> MAAEEGVASAASAGGSWGTAAMGRVLPMLLVPVPAEAMGQLGSRAQLRTQPEALGSLTAAGSLQVLSLTPGSRGGGRCCLEGPFWHFLWEDSRNSSTPTEKPKLLALGENYELLIYEFNLKDGRCDATILYSCSREALQKLIDDQDISISLLSLRILSFHNNTSLLFINKCVILHIIFPERDAAIRVLNCFTLPLPAQAVDMIIDTQLCRGILFVLSSLGWIYIFDVVDGTYVAHVDLALHKEDMCNEQQQEPAKISSFTSLKVSQDLDVAVIVSSSNSAVALNLNLYFRQ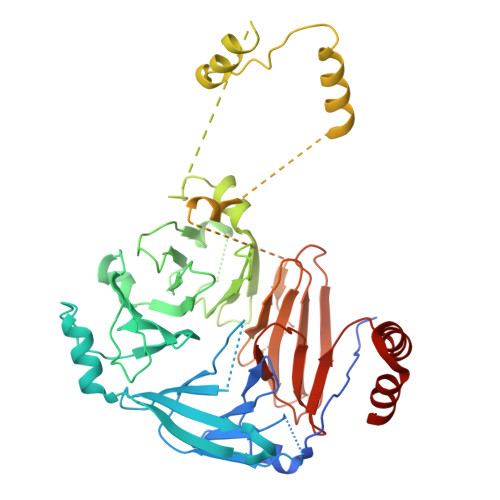HPGHLLCERILEDLPIQGPKGVDEDDPVNSAYNMKLAKFSFQIDRSWKAQLSSLNETIKNSKLEVSCCAPWFQDILHLESPESGNHSTSVQSWAFIPQDIMHGQYNVLQKDHAKTSDPGRSWKIMHISEQEEPIELKCVSVTGFTALFTWEVERMGYTITLWDLETQGMQCFSLGTKCIPVDSSGDQQLCFVLTENGLSLILFGLTQEEFLNRLMIHGSASTVDTLCHLNGWGR>GSAMDSSRRQYQEKYKQVEQYMSFHKLPADFRQKIHDYYEHRYQGKMFDEDSILGELNGPLREEIVNFNCRKLVASMPLFANADPNFVTAMLTKLKFEVFQPGDYIIREGTIGKKMYFIQHGVVSVLTKGNKEMKLSDGSYFGEICL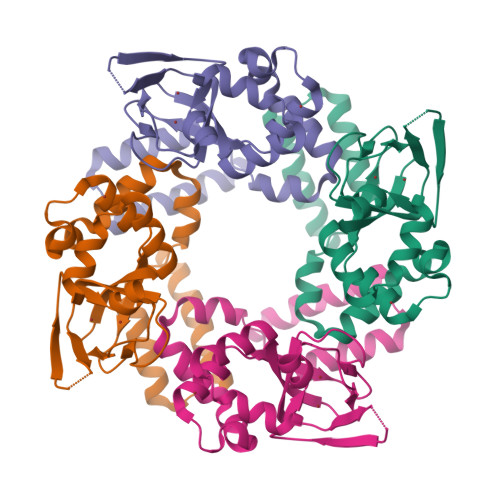LTRGRRTASVRADTYCRLYSLSVDNFNEVLEEYPMMRRAFETVAIDRLDRIGKKN[2x]>GAMDPEFMELRVGNRYRLGRKIGSGSFGDIYLGTDIAAGEEVAIKLECVKTKHPQLHIESKIYKMMQGGVGIPTIRWCGAEGDYNVMVMELLGPSLEDLFNFCSRKFSLKTVLLLADQMISRIEYIHSKNFIHRDVKPDNFLMGLGKKGNLVYIIDFGLAKKYRDARTHQHIPYRENKNLTGTARYASINTHLGIEQSRRDDLESLGYVLMYFNLGSLPWQGLKAATKRQKYERISEKKMSTPIEVLCKGYPSEFATYLNFCRSLRFDDKPDYSYLRQLFRNLFHRQGFSYDYVFDWNML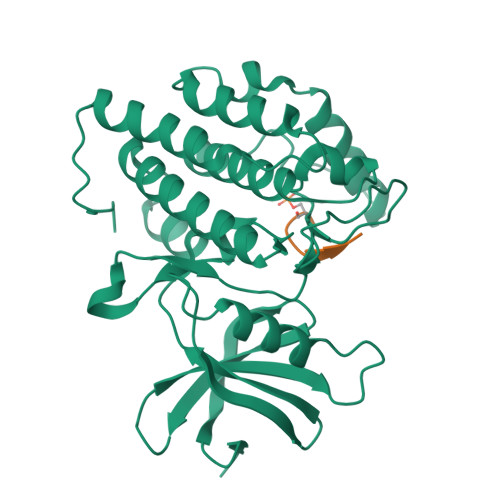K[2x];>[2x]VAERDSVMLGEIAPHHDY4-mercaptoidenecyclohexa-2,5-diene-1,2-dicarboxylic 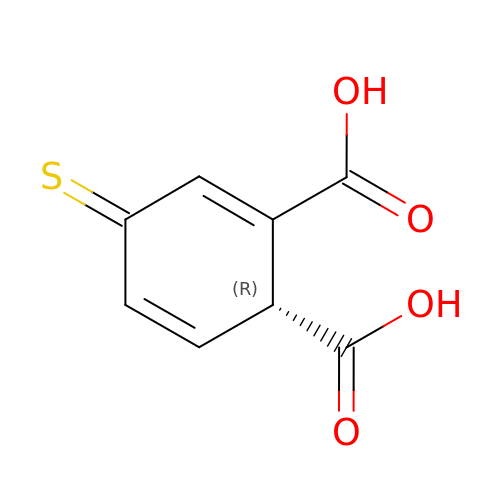acid | C8 H6 O4 S | KNBOUYAMGNHOJT-RXMQYKEDSA-N> MSLTGTDFHVGIVGLGSMGMGAARSCLRAGLSTWGADLNPQACANLLAEGACGAAASAREFAGVVDALVILVVNAAQVRQVLFGEDGVAHLMKPGSAVMVSSTISSADAQEIAAALTALNLNMLDAPVSGGAVKAAQGEMTVMASGSEAAFTRLKPVLDAVASNVYRISDTPGAGSTVKIIHQLLAGVHIAAAAEA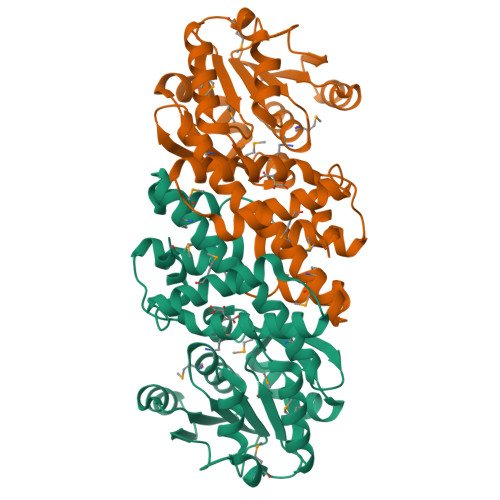MALAARAGIPLDVMYDVVTHAAGNSWMFENRMQHVVDGDYTPRSAVDIFVKDLGLVADTAKALRFPLPLASTALNMFTSASNAGYGKEDDSAVIKIFSGEGHHHHHH>[2x]GPLGSMAGTFKIHAYTEGGKPLRTIYLPKLLKKVFLDVVKPNTKKNLETCGILCGKLRQNAF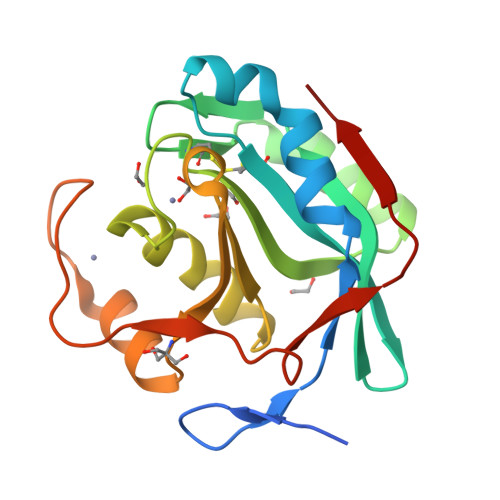FITHLVIPLQEATSDTCGTTDEASLFEFQDKHNLLTLGWIHTHPTQTCFMSSVDLHTHCSYQLMLPEAIAIVMAPSKNTSGIFRLLDPEGLQTIVKCRKPGLWHPHEGKVYTMVAQPGHVREINSKLQVVDLRVK8-[[(3R,4R)-3-[[1,1-bis(oxidanylidene)thian-4-yl]methoxy]piperidin-4-yl]amino]-3-methyl-5-(5-methylpyridin-3-yl)-1H-quinolin-2-one 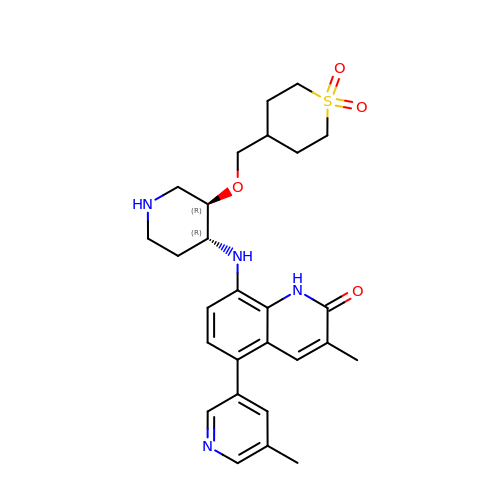| C27 H34 N4 O4 S | KXXIBIBXJMYWNL-ILBGXUMGSA-N>[23x]QVINTNSLSLITQNNINKNQSALSSSIERLSSGLRINSAKDDAAGQAIANRFTSNIKGLTQAARNANDGISVAQTTEGALSEINNNLQRIRELTVQASTGTNSDSDLDSIQDEIKSRLDEIDRVSGQTQFNGVNVLAKDGSMKIQVGANDGQTITIDLKKIDSDTLGLNGFNVNGKGETANTAATLKDMSGFTAAAAPGGTVGVTQYTDKSAVASSVDILNAVAGADGNKVTTSADVGFGTPAAAVTYTYNKDTNSYSAASDDISSANLAAFLNPQARDTTKATVTIGGKDQDVNIDKSGNLTAADDGAVLYMDATGNLTKNNAGGDTQ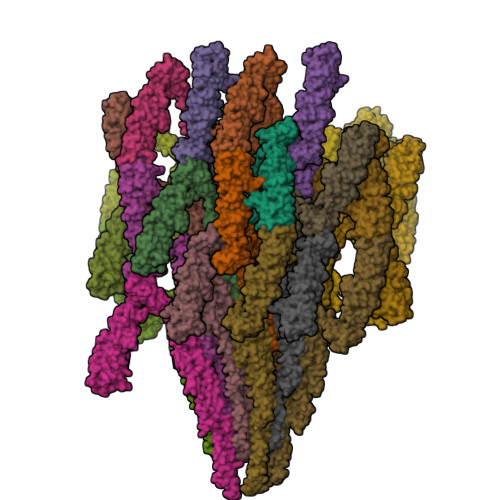ATLAKVATATGAKAATIQTDKGTFTSDGTAFDGASMSIDANTFANAVKNDTYTATVGAKTYSVTTGSAAADTAYMSNGVLSDTPPTYYAQADGSITTTEDAAAGKLVYKGSDGKLTTDTTSKAESTSDPLAALDDAISQIDKFRSSLGAVQNRLDSAVTNLNNTTTNLSEAQSRIQDADYATEVSNMSKAQIIQQAGNSVLAKANQVPQQVLSLLQG> GLVNFGNTCYCNSVLQALYFCRPFREKVLAYKSQPRKKESLLTCLADLFHSIATQKKKVGVIPPKKFITRLRKENELFDNYMQQDAHEFLNYLLNTIADILQEERKQEKQNGRLPNGNIDNENNNSTPDPTWVHEIFQGTLTNETRCLTCETISSKDEDFLDLSVDVEQNTSITHCLRGFSNTETLCSEYKYYCEECRSKQEAHKR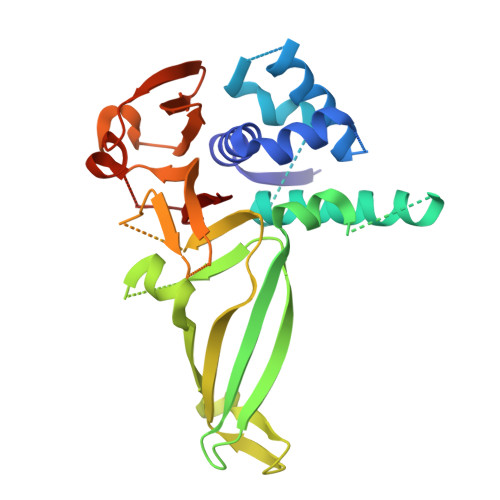MKVKKLPMILALHLKRFKYMDQLHRYTKLSYRVVFPLELRLFNTSGDATNPDRMYDLVAVVVHCGSGPNRGHYIAIVKSHDFWLLFDDDIVEKIDAQAIEEFYGLTSDISKNSESGYILFYQSRD6-benzylthio-2-chloropurine | C12 H9 Cl N4 S | 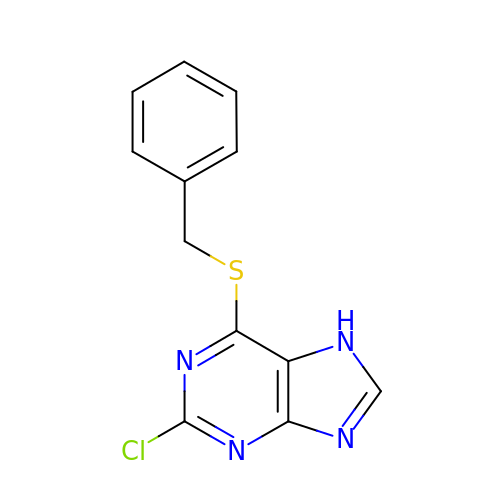CLBBDQGSXQEBIT-UHFFFAOYSA-N acetyl-oxa(dethia)-CoA | C23 H38 N7 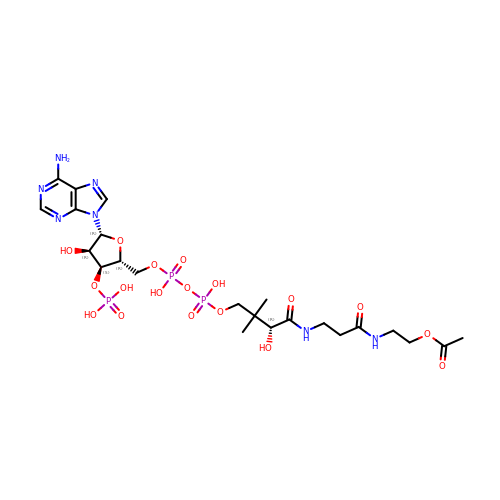O18 P3 | YTFJZNGIRMRBLL-ZSJPKINUSA-N> SWLLRLFESKLFDISMAISYLYNSKEPGVQAYIGNRLFCFRNEDVDFYLPQLLNMYIHMDEDVGDAIKPYIVHRCRQSINFSLQCALLLGAYSSDMHISTQRHSRGTKLRKLILSDELKPAHRKRELPSLSPAPDTGLSPSKRTHQRSKSDATASISLSSNLKRTASNPKVENEDEELSSSTESIDNSFSSPVRLAPEREFIKSLMAIGKRLATLPTKEQKTQRLISELSLLNHKLPARVWLPTAGFDHHVVRVPHTQAVVLNSKDKAPYLIYVEVLECENFDTTSVPARIPENRRDPEDPSAVALKEPWQEKVRRIREGSPYGHLPNWRLLSVIVKCGDDLRQELLAFQVLKQLQSIWEQERVPLWIKPYKILVISADSGMIEPVVNAVSIHQVKKQSQLSLLDYFLQEHGSYTTEAFLSAQRNFVQSCAGYCLVCYLLQVKDRHNGNILLDAEGHIIHIDFGFILSSSPRNLGFETSAFKLTTEFVDVMGGLDGDMFNYYKMLMLQGLIAARKHMDKVVQIVEIMQQGSQLPCFHGSSTIRNLKERFHMSMTEEQLQLLVEQMVDGSMRS;> GAMGSMGTRDDEYDYLFKVVLIGDSGVGKSNLLSRFTRNEFNLESKSTIGVEFATRSIQVDGK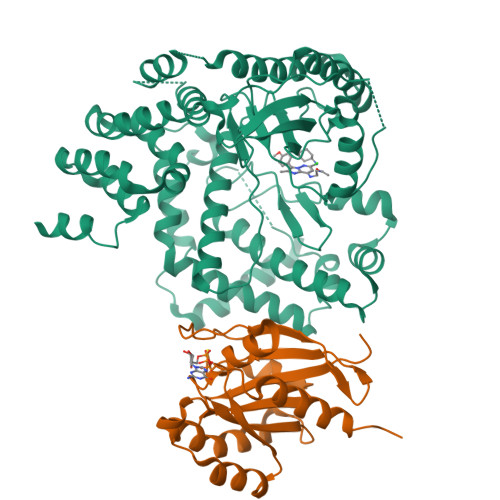TIKAQIWDTAGLERYRAITSAYYRGAVGALLVYDIAKHLTYENVERWLKELRDHADSNIVIMLVGNKSDLRHLRAVPTDEARAFAEKNGLSFIETSALDSTNVEAAFQTILTEIYRIVSQKQMSDRRENDMSPSNNVVPIHVPPTTENKPKVQCCQNI> MRSAQVYRWQIPMDAGVVLRDRRLKTRDGLYVCLREGEREGWGEISPLPGFSQETWEEAQSVL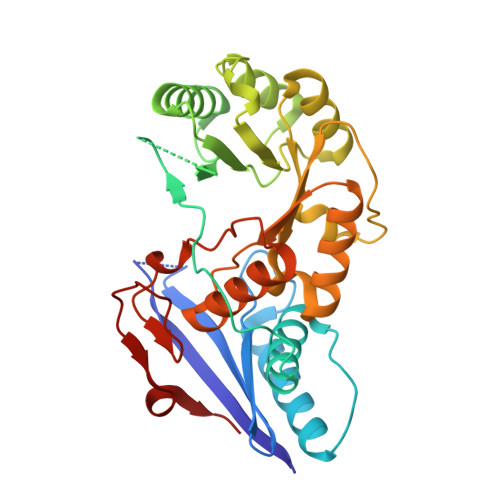LAWVNNWLAGDCELPQMPSVAFGVSCALAELTDTLPQAANYRAAPLCNGDPDDLILKLADMPGEKVAKVKVGLYEAVRDGMVVNLLLEAIPDLHLRLDANRAWTPLKGQQFAKYVNPDYRDRIAFLEEPCKTRDDSRAFARETGIAIAWDESLREPDFAFVAEEGVRAVVIKPTLTGSLEKVREQVQAAHALGLTAVISSSIESSLGLTQLARIAAWLTPDTIPGLDTLDLMQAQQVRRWPGSTLPVVEVDALERLL> DDDDKAMAGNFWQSSHY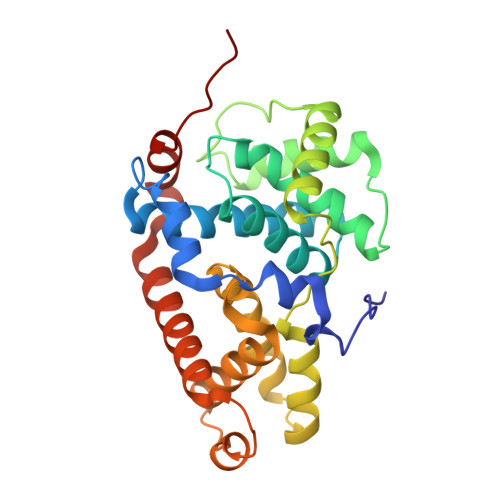LQWILDKQDLLKERQKDLKFLSEEEYWKLQIFFTNVIQALGEHLKLRQQVIATATVYFKRFYARYSLKSIDPVLMAPTCVFLASKVEEFGVVSNTRLIAAATSVLKTRFSYAFPKEFPYRMNHILECEFYLLELMDCCLIVYHPYRPLLQYVQDMGQEDMLLPLAWRIVNDTYRTDLCLLYPPFMIALACLHVACVVQQKDARQWFAELSVDMEKILEIIRVILKLYEQWKNFDERKEMATILSKMPKPKPPP>[2x]PKPINVRVTTMDAELEFAIQPNTTGKQLFDQVVKTIGLREVWYFGLHYVDNKGFPTWLKLDKKVSAQEVRKENPLQFKFRAKFYPEDVAEELIQDITQKLFFLQVKEGILSDEIYCPPETAVLLGSYAVQAKFGDYNKEVHKSGYLSSERLIPQ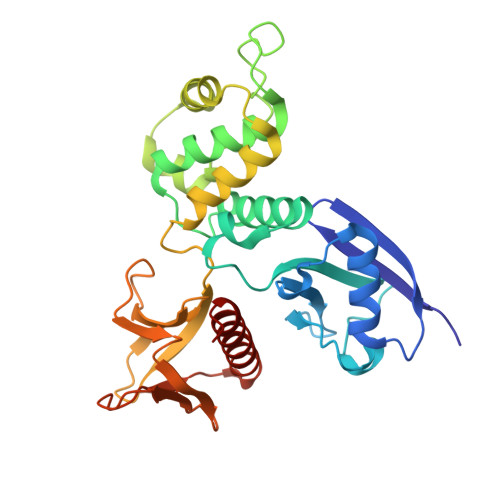RVMDQHKLTRDQWEDRIQVWHAEHRGMLKDNAMLEYLKIAQDLEMYGINYFEIKNKKGTDLWLGVDALGLNIYEKDDKLTPKIGFPWSEIRNISFNDKKFVIKPIDKKAPDFVFYAPRLRINKRILQLCMGNHELYMRRRKP When they were initially discovered, type III interferons (IFNλ1-3) were structurally and evolutionarily classified as members of the IL-10 superfamily of cytokines. Further investigation, though, revealed that they are functionally interferons (IFNs) with distinct roles in mucosal and innate immunity. While predicted to be structurally similar to IFNλ1-3, IFNλ4 shares only 28% amino acid sequence identity with its closest relative IFNλ3 and has a distinct biochemical composition resulting in IFNλ4 being one of the most positively-charged known cytokines (pI = 11.3). We next use protein engineering to overcome the affinity limitation for structural determination of the ternary IFNλ cytokine-receptor complex and determine the 72 kilodalton (kDa) structures of IFNλ4 as well as IFNλ3 in complex with IFNλR1 and an affinity-matured IL10Rβ via cryogenic electron microscopy (cryoEM).

Through extensive optimization of sample preparation, we successfully determined both ternary complexes using single-particle analysis to final resolutions of 3.26 Å for IFNλ4 and 3.00 Å for IFNλ3. B The structure of the IFNλ3 (blue) ternary complex solved in parallel with the IFNλ4 complex provides a frame of reference for differences in receptor engagement of IFNλR1 and IL10Rβ-A3. Overall, the structures of the IFNλ4:IFNλR1:IL10Rβ-A3 and IFNλ3:IFNλR1:IL10Rβ-A3 complexes are similar to the previously solved ternary complex of an engineered, high-affinity IFNλ3 (H11) with IFNλR1 and IL10Rβ27. Viewing the ligand from the front, IFNλ3 has a large acidic patch that engages with both IFNλR1 and IL10Rβ, but mostly the latter; while the acidic regions of the protein contacting IFNλR1 are mostly conserved, this same region for IFNλ4 at the IL10Rβ interface contains more basic and neutral residues. IFNλ3 and IFNλ4 make extensive contact with IFNλR1 and highlight the ability of the receptor to engage with basic residues, most notably Asp98 on IFNλR1 interacting with Arg47 of IFNλ4 and Lys21 of IFNλ3, which find themselves at similar locations and forming similar polar contacts at the interface. The importance of the hydrophobic residue network on IL10Rβ has been extensively described and consists of the Tyr59 residue in Loop 2, Tyr82 in Loop 3, and Tyr140 and Trp143 in Loop 527,36–39. These residues indeed form extensive contacts with IFNλ4 and IFNλ3, but in distinct orientations. Tyr82 engages spatially similar areas of IFNλ4 and IFNλ3 and in both cases is almost completely buried at the interface (>97%) but due to the differences in their surface charges, Tyr82 with IFNλ4 forms a hydrogen bond with the backbone nitrogen of Glu36 instead of the multiple hydrogen bonds formed with Ser11 and Ser13 on IFNλ3. Tyr59 in the IFNλ3 structure shares two hydrogen bonds with the ligand at Glu73 and Asp87, whereas there are no polar contacts shared with IFNλ4, indicating that the latter interaction is more hydrophobic in nature.

> GSMVPPPENVRMNSVNFKNILQWESPAFAKGQLTFTAQYLSYRIFQDKCMQTTLTECDFSSLSKYGDHTLRVRAEFADEHSDWVQITFCPVDDTIIGPPGMQVEVLADSLHMRFLAPKIENEYETWTMKDMYNSWTYNVQYWKQGTDEKFQITPQYDFEVLRNLEPRTTYCVQVRGFLPDRNKAGEWSEPVCEQTTHDETVPSAAAHHHHHH;> RPRLAPPQNVTLLSQNFSVYLTWLPGLGNPQDVTYFVAYQSSPTRRRWREVEECAGTKELLCSMMCLKKQDLYNKFKGRVRTVSPSSKSPWVESEYLDYLFEVEPAPPVLVLTQTEEILSANATYQLPPCMPPLDLKYEVAFWKEGAGNKTLFPVTPHGQPVQITLQPAASEHHCLSARTIYTFSVPKYSKFSKPTCFLLEVPEANAAA;> GSARGCHIAQFKSLSPQELQAFKRAKDALEESLLLKDCKCRSRLFPRTWDLRQLQVRERPVALEAELALTLKVLEATADTDPALGDVLDQPLHTLHHILSQLRACIQPQPTAGPRTRGRLHHWLHRLQEAPKKESPGCLEASVTFNLFRLLTRDLNCVASGDLCVAAAHHHHHHHH> 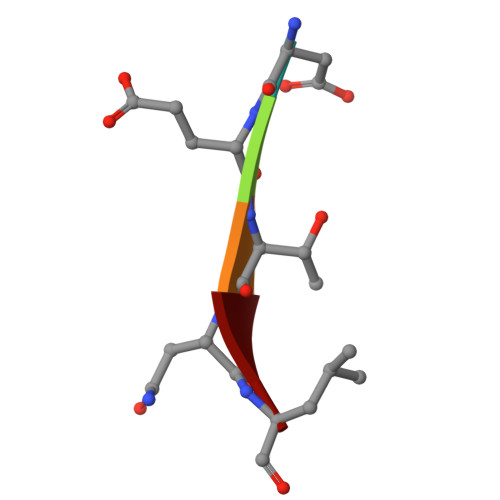DETNL>[4x]AGRKMDIVIRAAWQLFLEQGFSATSMDAIAKAA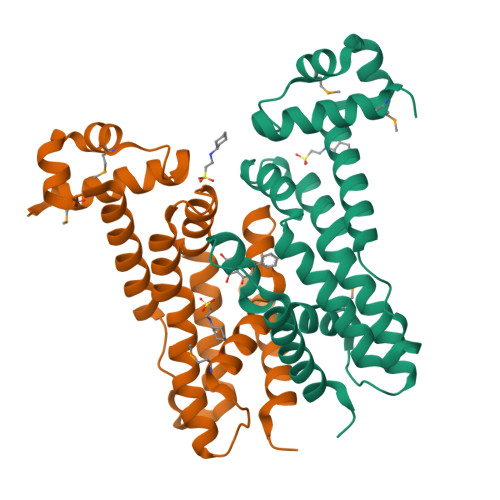GVSKATLYAYFPSKEALFASLIVAECESLQRDLPVPKLSAGLSEALRDFARQYLHTFIHRKDVAFVRIIANESGRFPVLARLFYESGPEATIRRLAQFLEEARAARVLEFDDPMEAANQFLSLVRGELPLLIVLGLSDLTEEAIEQEIEAGLKFFLKACQPR> GPHMELDQVVDVPAMLEVLEKEAVSLS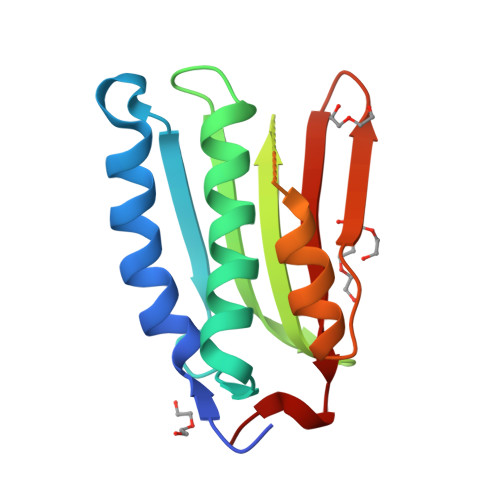GEAQHKLHFEVDKSLKVLADEDQLRSAISNLVYNAVKYTPPGAQIDVRWYRTGKGACLEVEDKGEGIEPQHLHRLTERFYRVDKARSRDTGGSGLGLAIVKHALAHHDTHLDIYSKVGVGSKFSFVLPKRLVAK> GSHMGSPEEYRELVVSLRV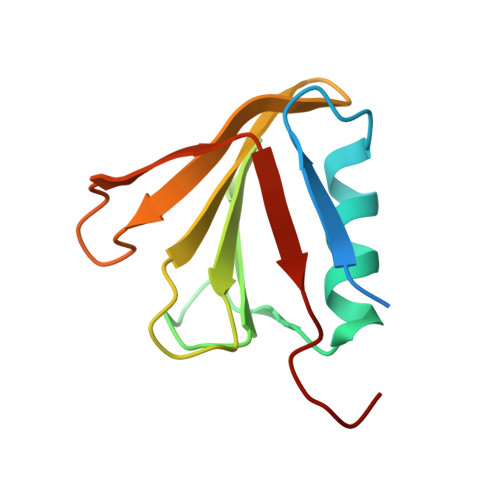GMEIERNALLRRLVDIQYDRNDIDFRRGTFRVRGDVVEIFPASRDEHCIRVEFFGDEIERIREVDALTGEVLGEREHVAIFPASHFV> GSKRDHHQFQGRLSNHGTSSSSSSISKDKMMMVKKEEDGGGNMDDELLAVLGYKVRSSEMAEVALKLEQLETMMSNVQEDGLSHLATDTVHYNPSELYSWLDNMLSELNPPPLPASSNGLDPVLPSPEICGFPASDYDLKVIPGNAIYQFPAIDSSSSSNNQNKRLKSCSSPDSMVTSTSTGTQIGGVIGTTVTTTTTTTTAAGESTRSVILVDSQENGVRLVHALMACAEAIQQNNLTLAEALVKQIGCLAVSQAGAMRKVATYFAEALARRIYRLSPPQNQIDHCLSDTLQMHFYETCPYLKFAHFTANQAILEAFEGKKRVHVIDFSMNQGLQWPALMQALALREGGPPTFRLTGIGPPAPDNSDHLHEVGCKLAQLAEAIHVEFEYRGFVANSLADLDASMLELRPSDTEAVAVNSVFELHKLLGRPGGIEKVLGVVKQIKPVIFTVVEQESNHNGPVFLDRFTESLHYYSTLFDSLEGVPNSQDKVMSEVYLGKQICNLVACEGPDRVERHETLSQWGNRFGSSGLAPAHLGSNAFKQASMLLSVFNSGQGYRVEESNGCLMLGWHTRPLITTSAWKLSTAAY;> GSMAA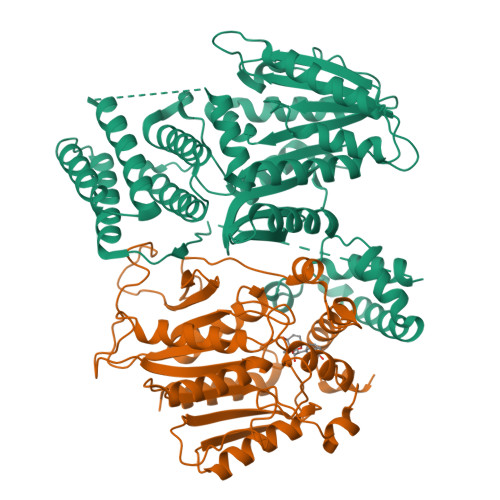SDEVNLIESRTVVPLNTWVLISNFKVAYNILRRPDGTFNRHLAEYLDRKVTANANPVDGVFSFDVLIDRRINLLSRVYRPAYADQEQPPSILDLEKPVDGDIVPVILFFHGGSFAHSSANSAIYDTLCRRLVGLCKCVVVSVNYRRAPENPYPCAYDDGWIALNWVNSRSWLKSKKDSKVHIFLAGDSSGGNIAHNVALRAGESGIDVLGNILLNPMFGGNERTESEKSLDGKYFVTVRDRDWYWKAFLPEGEDREHPACNPFSPRGKSLEGVSFPKSLVVVAGLDLIRDWQLAYAEGLKKAGQEVKLMHLEKATVGFYLLPNNNHFHNVMDEISAFVNAEC>[2x]MEKYQALLAN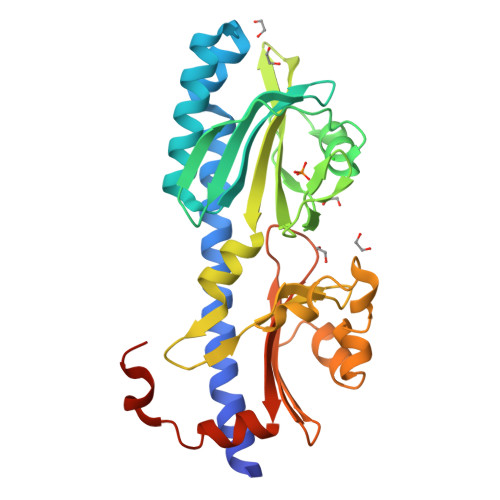NVENTAKEALHQLAYTGREYNNIQDQIETISDLLGHSQSLYDYLREPSKANLTILENMWSSVARNQKLYKQIRFLDTSGTEKVRIKYDFKTSIAGPSLILRDKSAREYFKYAQSLDNEQISAWGIELERDKGELVYPLSPSLRILMPISVNDVRQGYLVLNVDIEYLSSLLNYSPVRDFHIELVKHKGFYIASPDESRLYGDIIPERSQFNFSNMYPDIWPRVVSEQAGYSYSGEHLIAFSSIKFVSNEPLHLIIDLSNEQLSKRATRDINDLIQESLEHHHHHH2-[1-[3-[(4~{S})-6-azanyl-5-cyano-3-methyl-4-propan-2-yl-2~{H}-pyrano[2,3-c]pyrazol-4-yl]-5-(trifluoromethyl)phenyl]piperidin-4-yl]ethanoic acid | C25 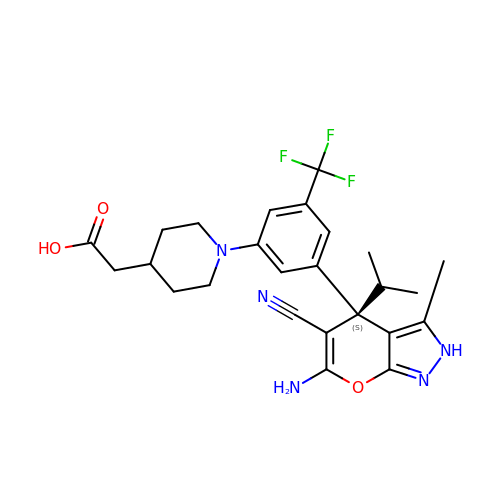H28 F3 N5 O3 | UHPFIFHQJWKZHI-DEOSSOPVSA-N> GAPATVTEQGEDITSKKDRGVLKIVKRVGNGEETPMIGDKVYVHYKGKLSNGKKFDSSHDRNEPFVFSLGKGQVIKAWDIGVATMKKGEICHLLCKPEYAYGSAGSLPKIPSNATLFFEIELLDFKGE

A typical example is the family of FK506‐binding proteins (FKBPs) that possess a highly conserved binding pocket but have diverged to perform diverse biological functions. The larger homolog FKBP51 is a regulator of glucocorticoid receptor (GR) signaling and has emerged as a potential target for depression, obesity‐induced diabetes and chronic pain. The most advanced FKBP51 ligands are compounds of the SAFit class (Selective Antagonists of FKBP51 by induced fit), which bind to a transient binding pocket unavailable to FKBP52 and are up to 10 000‐fold selective for FKBP51 over FKBP52. During a macrocyclization pilot study, we observed that many of these macrocyclic analogs have unanticipated and unprecedented preference for FKBP51 over FKBP12 and FKBP12.6.

The glycine derivative 13 a had an affinity of 2.3 μm, which gradually increased with increasing substitution (13 b (d‐Ala): 1.0 μm, 13 c (Aib): 0.29 μm). The affinity of 13 a and d for FKBP51 was confirmed by isothermal calorimetry (ITC), yielding an enthalpy‐driven K d=3.6 μm ±0.9 μm for 13 a and K d=0.6 μm ±0.1 μm for 13 d, respectively. As intended, the interactions of the pipecolate, the A‐ and B‐rings, as well as the cyclohexyl group with FKBP51 were completely conserved in comparison to previous FKBP51‐SAFit co‐crystal structures. This includes a displacement of F67, which is responsible for the strong selectivity vs. FKBP52 of SAFit‐like ligands. Strikingly, we observed that the carbonyl group of 13 a, 13 d and 13 h displaced D68 and replaced it as a hydrogen bond acceptor for the ϵ‐hydroxy group of Y57. The rearrangement of the β3b strand is stabilized by an inward flip of H71, which partially replaces S70 and substitutes the former as a hydrogen bond donor for the backbone carbonyl of Y57. Intriguingly, H71 is replaced in FKBP12 and FKBP12.6 by an arginine (R40 in FKBP12/12.6 numbering), which can be expected to be less efficient in stabilizing the 13 a‐binding conformation, providing a molecular rationale for the discrimination vs. FKBP12/12.6 observed for the macrocycles. In this particular case, the macrocycles provide the scaffold for the proper positioning of the key carbonyl group that displaces Asp68, which was not possible in the linear analogs.>MGTRDDEYDYLFKVVLIGDSGVGKSNLLSRFTRNEFNLESKSTIGVEFATRSIQVDGKTIKAQIWDTAGLERYRAITSAYYRGAVGALLVYDIAKHLTYENVERWLKELRDHADSNIVIMLVGNKSDLRHLRAVPTDEARAFAEKNGLSFIETSALDSTNVEAAF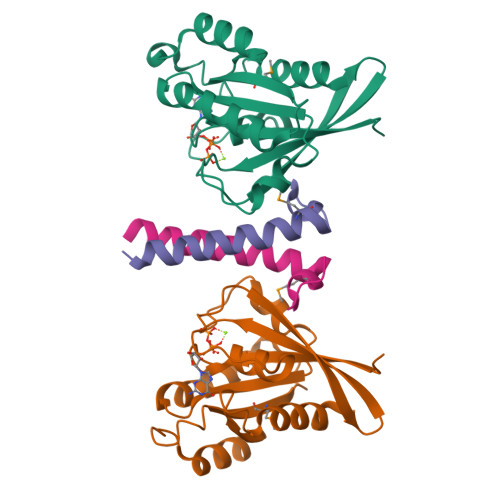QTILTEIY[2x];>GAMAAKFRASNIMPSSSFHMSPTSNEDLRKIPDSNPFDATAGYRSLTYEEVLQELVKHKELLRRKDTHIRELEDYIDNLLVRVMEETPSILRVPYEPSRKAGKFSNS[2x]N-cyclopropyl-1-(4-phenylpyridin-3-yl)piperidine-4-carboxamide | C20 H23 N3 O | 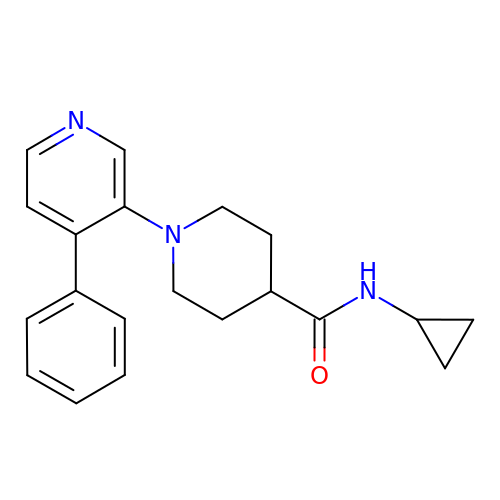IEDSUIIRTVCTDM-UHFFFAOYSA-N1-(6-CYANO-3-PYRIDYLCARBONYL)-5',8'-DIFLUOROSPIRO[PIPERIDINE-4,2'(1'H)-QUINAZOLINE]-4'-AMINE | C19 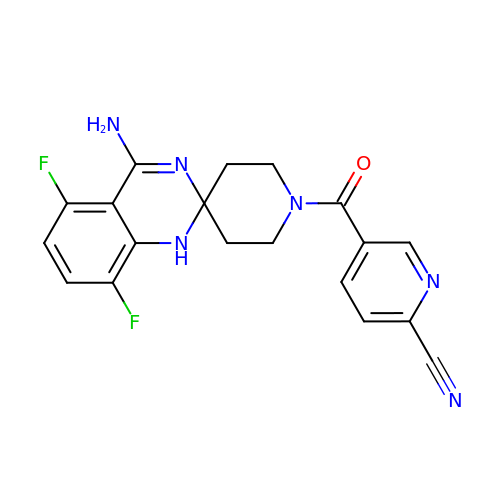H16 F2 N6 O | GIZYIOOBBUHOBS-UHFFFAOYSA-N1-[2-(4-METHYLPHENOXY)ETHYL]-2-(2-PHENOXYETHYLSULFANYL)BENZIMIDAZOLE | C24 H24 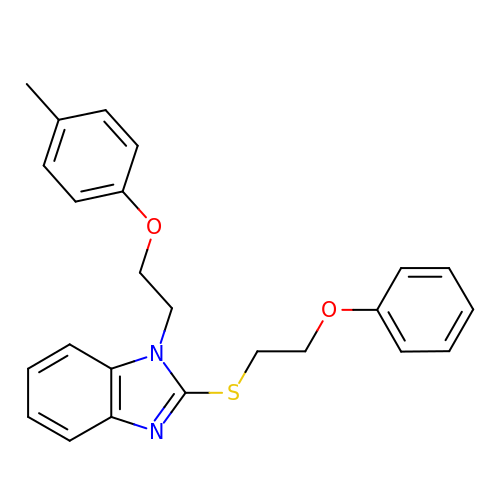N2 O2 S | PNCBJXVNIRRHJP-UHFFFAOYSA-N> MNQQKSLTLIVALTTSYGIGRSNSLPWKLKKEISYFKRVTSFVPTFDSFESMNVVLMGRKTWESIPLQFRPLKGRINVVITRNESLDLGNGIHSAKSLDHALELLYRTYGSESSVQINRIFVIGG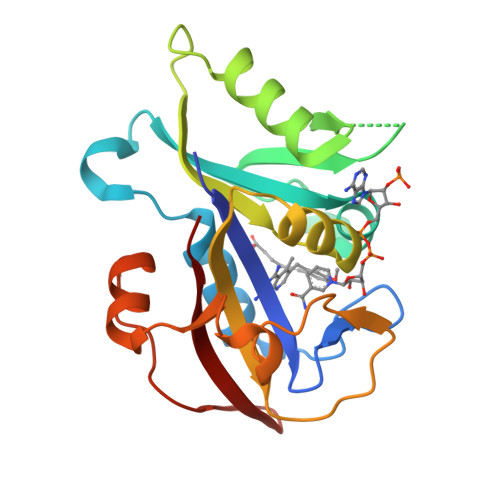AQLYKAAMDHPKLDRIMATIIYKDIHCDVFFPLKFRDKEWSSVWKKEKHSDLESWVGTKVPHGKINEDGFDYEFEMWTRDL>MDWHIAKHYDDILYYKAGGIAKIVINRPHKRNAFRPQTVFELYDAFCNAREDNRIGVVLLTGAGPHSDGKYAFCSGGDQSVRGEGGYID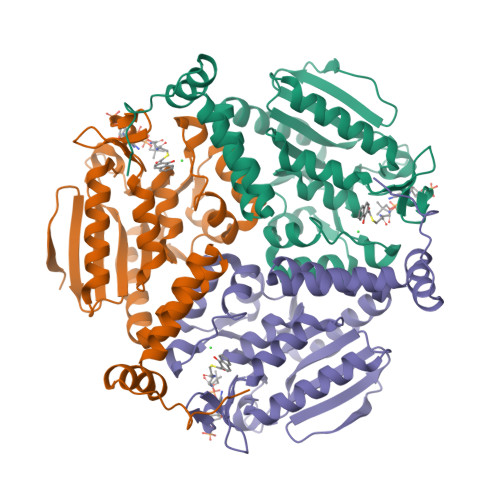DQGTPRLNVLDLQRLIRSMPKVVIALVAGYAIGGGHVLHLVCDLTIAADNAIFGQTGPKVGSFDGGFGSSYLARIVGQKKAREIWYLCRQYSAQEAERMGMVNTVVPVDRLEEEGIQWAKEILSKSPLAIRCLKAAFNADCDGQAGLQELAGNATLLYYMTEEGSEGKQAFLEKRPPDFSQYPWLP[9x]>[2x]GPLGSMSLQEKLLTYYRNRAAIPAGEQARAKQAAVDICAELRSFLRAKLPDMPLRDMYLSGSLYDDLQVVTADHIQLIVPLVLE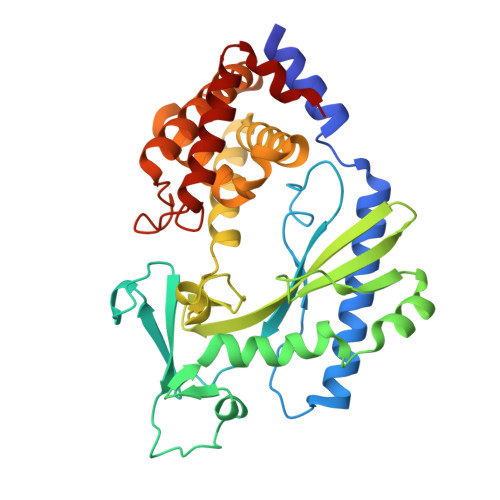QNLWSCIPGEDTIMNVPGFFLVRRENPEYFPRGSSYWDRCVVGGYLSPKTVADTFEKVVAGSINWPAIGSLLDYVIRPAPPPEALTLEVQYERDKHLFIDFLPSVTLGDTVLVAKPHRLAQYDNLWRLSLRPAETARLRALDQADSGCRSLCLKILKAICKSTPALGHLTASQLTNVILHLAQEEADWSPDMLADRFLQALRGLISYLEAGVLPSALNPKVNLFAELTPEEIDELGYTLYCSLSEPEVLLQT> ENKFITKDDEVIDYIYGKISPLFALQYIRKIDLKHVFEYDYHFE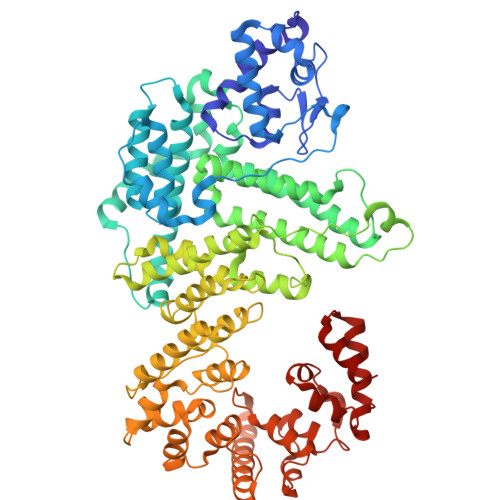VNGTVVRHKNKGFGYMERFFELKESCDERSKLSKKQYERFNALFNFFEKNGVICMAKDAGTLNTSIEINSLAYHGKYDVMKKFIEEQSVSIEDDYKKAFFLACLGRWEESYDLYSNIILNSIDESNGCVYYLSQINRYRIYQSITQAVTQFNGLGLLTFGRHYKPFTDEFLARIEREMTNFNIDDLFNGMPFEFQKKYKILEFLSDNQFLYDDTVKLFELTNKVRSEMSEGSYSFGMSSDIVVLLRLYDNLRFLYENCLWSVSFHEFHQYIRNSMSLLIEKAEYERTRDIDELGFSFFGKKSGFFMEYYDFVNISRHFKIDDIKNLERSCSIDKIRFGEQEKIEEYLVGIAEEITKQFSANGMNVVFYTQFISEAKAALYFAKYVKLSEEGLGKIVKALLFYFPERDLDIGKRYVWLERLTKCNELPKSIISIIDDFLVLQAEKHIDQNYSEVSSNGLYSRDYGALIKHFEKNFISKRLSEITLCLTQDKQKQIDFLFKLLPLLSTNAKSHLLSFKSVENINDLMNGIRIGLIDEFTPEHEELIIEYLETRKVNYIVEKEKGIQTFSSNDYMSTFGIWYFLEEINNSKMEEFIGMDDQYDFFVDPENFDYKKFIPSWLKNYNDKLLGKIAGNKHMKHHVIEVLKERVKNSNDKRYLEILMNYFI4-ethylbenzenesulfonamide 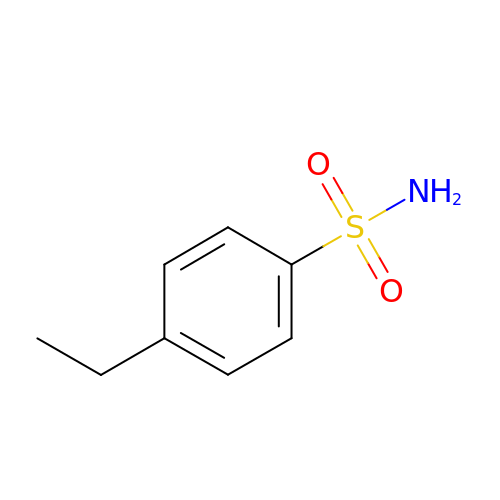| C8 H11 N O2 S | MLTGAVXHWSDGIS-UHFFFAOYSA-N5-butylpyridine-2-carboxylic acid | C10 H13 N O2 | 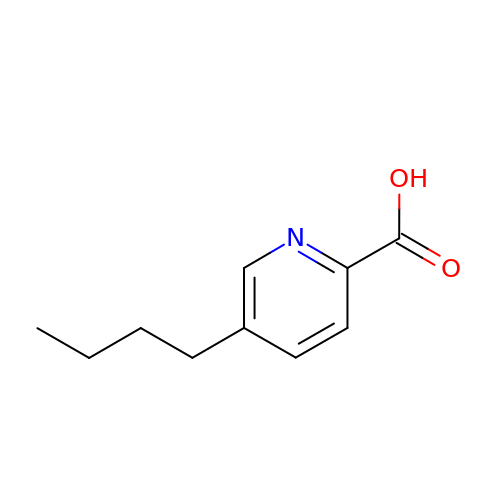DGMPVYSXXIOGJY-UHFFFAOYSA-N> MSNTYQKRKASKEYGLYNQCKKLNDDELFRLLDDHNSL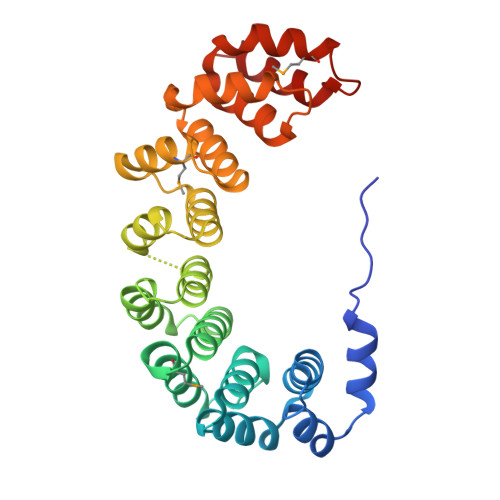KRISSARVLQLRGGQDAVRLAIEFCSDKNYIRRDIGAFILGQIKICKKCEDNVFNILNNMALNDKSACVRATAIESTAQRCKKNPIYSPKIVEQSQITAFDKSTNVRRATAFAISVINDKATIPLLINLLKDPNGDVRNWAAFAININKYDNSDIRDCFVEMLQDKNEEVRIEAIIGLSYRKDKRVLSVLCDELKKNTVYDDIIEAAGELGDKTLLPVLDTMLYKFDDNEIITSAIDKLKRS>KTISFNFNQFHQNEEQLKLQRDARISSNSVLELTKVVNGVPTWNSTGRALYAKPVQVWDSTTGNVASFETRFSFSIRQPFPRPHPADGLVFFIAPPNTQTGEGGGYFGIYNPLSPYPFVAVEFDTFRNTWDPQIPHIGIDVNSVISTKTVPFTLDNGGIANVVIKYD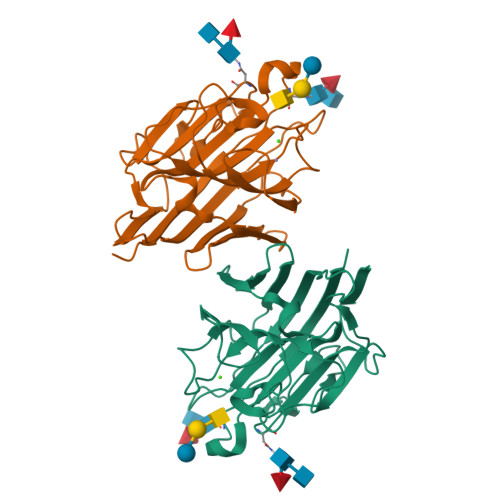ASTKILHVVLVFPSLGTIYTIADIVDLKQVLPESVNVGFSAATGDPSGKQRNATETHDILSWSFSASLPG[4x]> GSHMLEQIKNNFTESIQTQIAASELLGPSIEHAGMMMVQCLLGGNK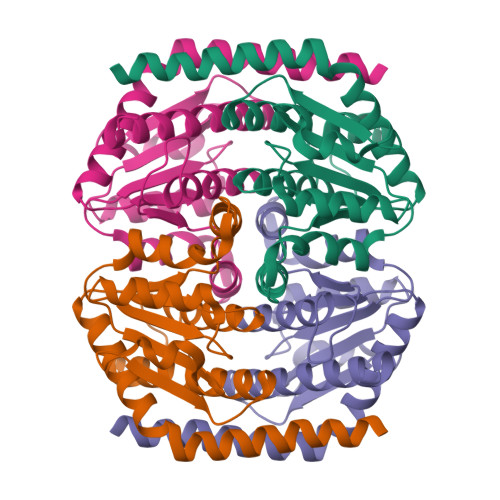IISCGNGGSAGHAQHFCAQLLNKYETERPSLPAISLNSDISTITSIANDYQYDEVFSKQIRALGHNGDVLLAISTSGNSRNVVKAIESAVSRDIPIIALTGFDGGDISGLLGEGDVEIRVPSARTSRIQEVHLVVLHSLCEIIDTTLFPQGDS> MHHHHHHSSGRENLYFQGNAVLTWNNEILPNWETMWCSRKVRDLWWQGIPPSVRGKVWSLAIGNELNITHELFDICLARAKERWRSLSTGGSEVENEDAGFSA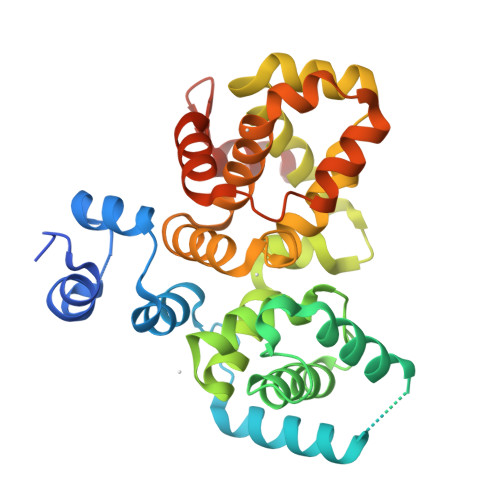ADREASLELIKLDISRTFPNLCIFQQGGPYHDMLHSILGAYTCYRPDVGYVQGMSFIAAVLILNLDTADAFIAFSNLLNKPCQMAFFRVDHGLMLTYFAAFEVFFEENLPKLFAHFKKNNLTPDIYLIDWIFTLYSKSLPLDLACRIWDVFCRDGEEFLFRTALGILKLFEDILTKMDFIHMAQFLTRLPEDLPAEELFASIATIQMQSRNKKWAQVLTALQKDSREMEKG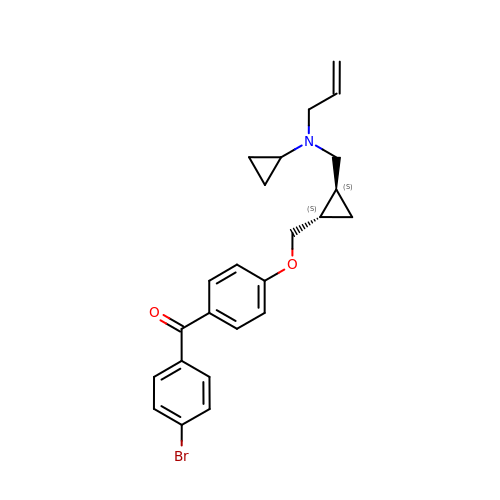{4-[((1S,2S)-2-{[ALLYL(CYCLOPROPYL)AMINO]METHYL}CYCLOPROPYL)METHOXY]PHENYL}(4-BROMOPHENYL)METHANONE | C24 H26 Br N O2 | ICPGWJRDLWZVKA-WOJBJXKFSA-N>MFKRETKDFINIDPLQTGGKLTEEARQALLEWGDGYSVCDFCTTGRLDEIKTPPIHDFIHNQLPKFLGCDVARVTNGAREAKFAVMHSLAKKDAWVVMDENCHYSSYVAAERAGLNIALVPKTDYPDYAITPENFAQTIEETKKRGEVVLALITYPDGNYGNLPDVKKIAKVCSEYDVPLLVNGAYAIGRMPVSLKEIGADFIVGSGHKSMAASGPIGVMGMKEEWAEIVLRRSEKYKNKEVELLGCTARGATIITLMA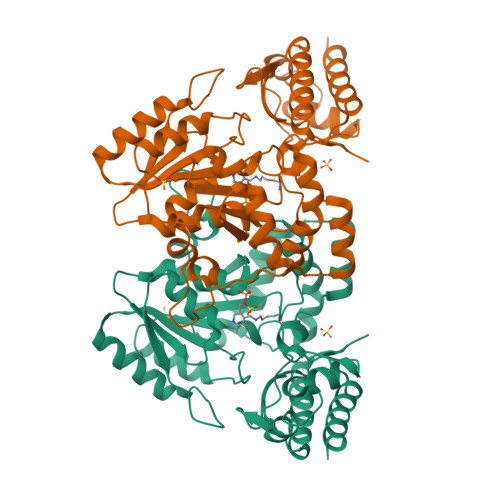SFPHVRERIKRWDEEVEKARRFAAEMEKLGIKQLGDNPHNHDLMFFHAEVLYEISKKAKGGRFFLYRELKSRKIHGIKPGLTRYFKLSTYGLSDEEVDYVLNAFKEIIEKYS[2x]>GCCSDPRCNMNNPDYC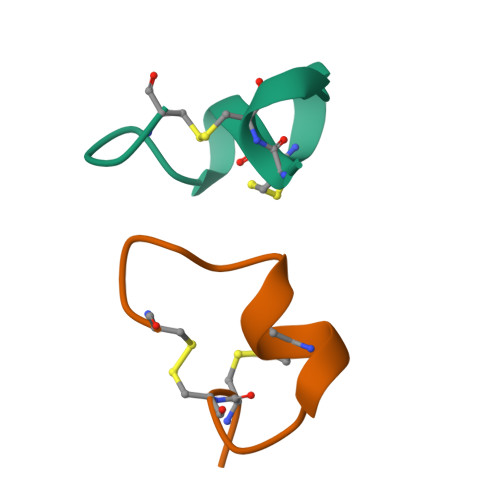X[2x]>GPLGSPEFMSVYHIKWIQWKEENTPIITQNENGPCPLLAILNVLLLAWKVKLPPMMEIITAEQLMEYLGDYMLDAKPKEISEIQRLNYEQNMSDAMAILHKLQTGLDVNVRFTGVRVFEYTPECIVFDLLDIPLYHGWLVDPQIDDIVKAVGNCSYNQLVEKIISCKQSDNSELVSEGFVAEQFLNNTATQLTYHGLCELTSTVQEGELCVFFRNNHFSTMTKYKGQLYLLVTDQGFLTEEKVVWESLHNVDGDGNFCDSEFHLRPPSDPETV[4x]

MINDY1 and MINDY2 are members of the MINDY family of deubiquitinases (DUBs) that have exquisite specificity for cleaving K48-polyUb, yet we have a poor understanding of their catalytic mechanism. Here, we analyze the crystal structures of MINDY1 and MINDY2 alone and in complex with monoUb, di-, and penta-K48-polyUb, identifying 5 distinct Ub binding sites in the catalytic domain that explain how these DUBs sense both Ub chain length and linkage type to cleave K48-polyUb chains. The activity of MINDY1/2 is inhibited by the Cys-loop, and we find that substrate interaction relieves autoinhibition to activate these DUBs. We also find that MINDY1/2 use a non-canonical catalytic triad composed of Cys-His-Thr.

In MINDY1 and MINDY2, a flexible loop (T130 to P138 in MINDY1 and T259 to P267 in MINDY2) connects β2 to α1, which we term the Cys loop since the catalytic cysteine sits at its base. In the apo-form of the DUB, this Cys loop occludes the catalytic center and would sterically hinder positioning of the scissile bond across the active site. The only significant change is in the Cys loop that undergoes significant remodeling, during which several hydrogen bonds are broken, accompanied by the formation of new bonds. This extensive interaction network and remodeling of the Cys loop is also observed in MINDY2, and when restructured, the Cys loop no longer impedes Ub binding. In contrast, in MINDY2apo, the catalytic H448 is flipped out, and Q260 is not able to form a hydrogen bond. However, the binding of Ubprox brings H448 closer to the catalytic C266 to form a productive active site. For both MINDY2 apo and MINDY2∼Ub complex, computed data from the models yielded good agreement with the experiment, confirming the two structures in solution.> MMTVLEDMLRKTRNGKVHMTLIDPGAKPPQECARIAEEAEMAGTDFIMVGGSTDIDSRAMDEAISAIKAKTDLKVIIFPGSSLMISPKADAIFFMSLLNSGSLEYVVGHQVKAAIPLSAMKIEKIPMAYLVFDPGMTVGRVGKAHLIPRDDEKTALSYALAAQYFGFRLVYFEAGSGSPYHVGENVVRRVKQELDIPVIVGGGIRTPEAAKALAQAGADMIVTGTIAERSVNV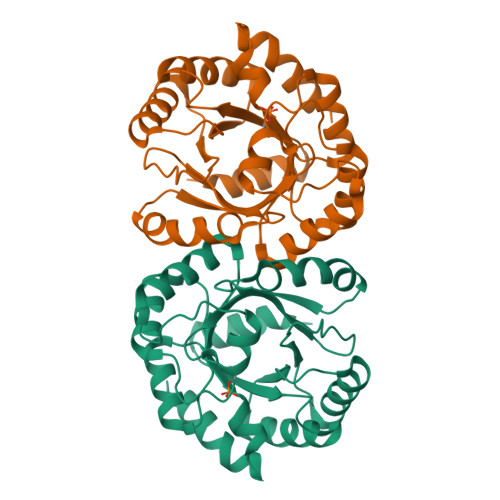YEALHPIVESIKEVGISKIQ> MERPESELIRQSWRVVSRSPLEHGTVLFARLFALEPSLLPLFQYNGRQFSSPEDSLSSPEFLDHIRKVMLVIDAAVTNVEDLSSLEEYL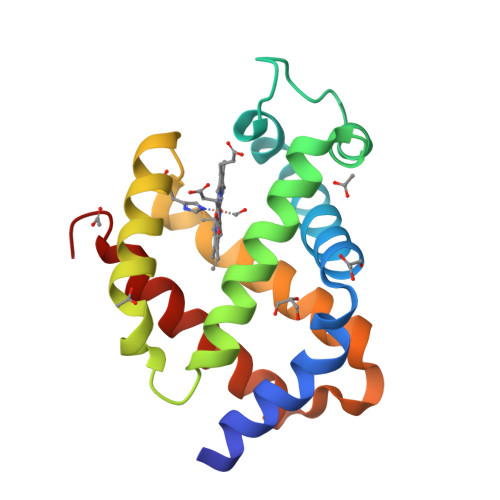TSLGRKHRAVGVRLSSFSTVGESLLYMLEKSLGPDFTPATRTAWSRLYGAVVQAMSRGWDG> MDLLYTLVILFYLGVAGLLVYLVLVQEPKQGAGDLMGGSA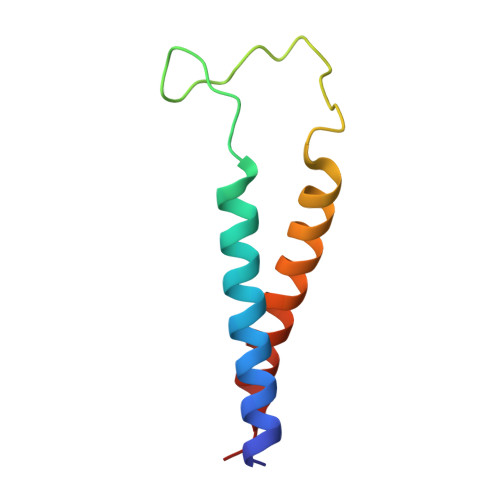DLFSARGVTGGLYRLTVILGVVFAALALVIGLWPR>[2x]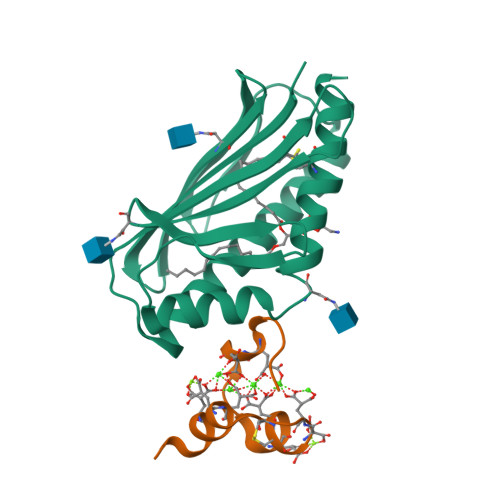SQDASDGLQRLHMLQISYFRDPYHVWYQGNASLGGHLTHVLEGPDTNTTIIQLQPLQEPESWARTQSGLQSYLLQFHGLVRLVHQERTLAFPLTIRCFLGCELPPEGSRAHVFFEVAVNGSSFVSFRPERALWQADTQVTSGVVTFTLQQLNAYNRTRYELREFLEDTCVQYVQKHISAENTKGSQTSRSYTS;>[2x]ANSFLEELRHSSLERECIEEICDFEEAKEIFQN>[2x]GFDYDVVVVGGGFAGATAARECGLQGYRTLLLEARSRLGGRTFTSRFAGQEIELGGTWVHWLQPHVWAEMQRYGLGVVEDPLTNLDKTLIMYNDGIVESISPDEF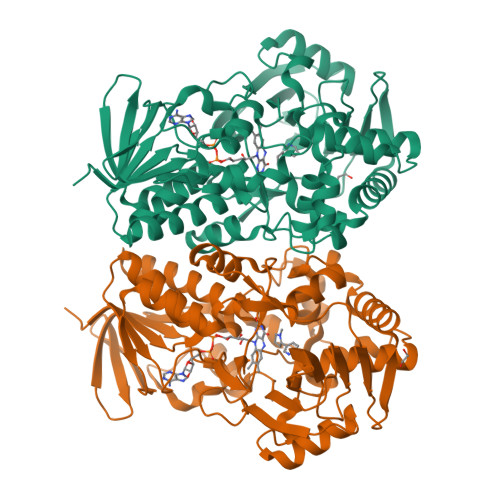GKNIRIAFEKLCHDAWEVFPRPHEPMFTERARELDKSSVLDRIKTLGLSRLQQAQINSYMALYAGETTDKFGLPGVLKLFACGGWNYDAFMDTETHYRIQGGTIGLINAMLTDSGAEVRMSVPVTAVEQVNGGVKIKTDDDEIITAGVVVMTVPLNTYKHIDFTPALSKGKQRFIKEGQLSKGAKLYVHVKQNLGRVFAFADEQQPLNWVQTRDYSDELGTILSITIARKETIDVNDRDAVTREVQKMFPGVEVLGTAAYDWTADPFSLGAWAAYGVGQLSRLKDLQAAEGRIVFAGAETSNGWHASIDGAVESGLRAGREVKQLLS> MSNLSGTDKSVILLMTIGEDRAAEVFKHLSTREVQALSTAMANVRQISNKQLTDVLSEFEQEAEQFAALNINANEYLRSVLVKALGEERASSLLEDILETR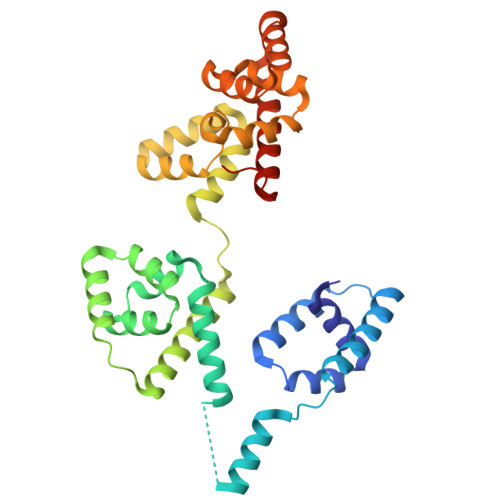DTTSGIETLNFMEPQSAADLIRDEHPQIIATILVHLKRSQAADILALFDERLRHDVMLRIATFGGVQPAALAELTEVLNGLLDGQNLKRSKMGGVRTAAEIINLMKTQQEEAVITAVREFDGELAQKIIDEMFLFENLVDVDDRSIQRLLQEVDSESLLIALKGAEPPLREKFLRNMSQRAADILRDDLANRGPVRLSQVENEQKAILLIVRRLAETGEMVIGSGEDTYV>[2x]MDKPILKDSMKLFEALGTIKSRSMFGGFGLF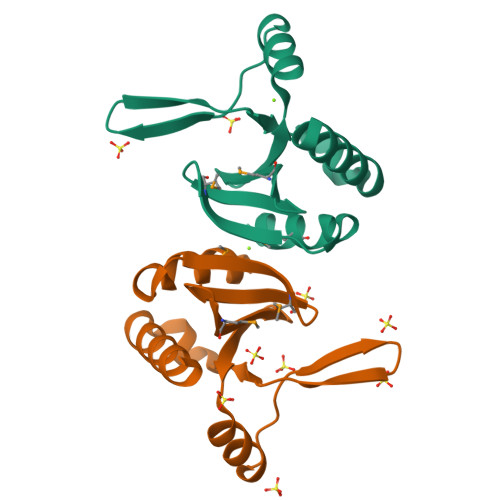ADETMFALVVNNQLHIRADQQTSSDFETQGLKPYVYKKRGFPVVTKYYAISSELWESSDRLIEVAKKSLENAKL Norovirus capsid displays an icosahedral symmetry that is composed of 180 copies of a single major structural protein, the capsid protein (VP1), which organize into 90 dimers. Each VP1 can be divided into two major domains, the N-terminal shell (S) and the C-terminal protruding (P) domains, linked by a short hinge. The P domain is further divided into P1 and P2 subdomains, forming the leg and the head of the protruding P dimer, respectively. Expression of the S domain alone formed smooth, thin-layer S particles without the protruding structures, while production of P domain in vitro resulted in P dimer, P particle, and small P particle. Functional analyses showed that the P dimer and the P particle, but not the S particle, bind to histo-blood group antigens (HBGAs), the host susceptible factors of noroviruses (see below), indicating that the P domain is the HBGA binding domain.

The P domain of VA207 (amino acid 222 to 537) was expressed in E. coli and the HBGA binding profile of the resulting P protein was verified (data not shown) before being used in the crystallography study. The crystal of the native P protein of VA207 belongs to space group of P21212 and contains a homodimer of P protein in an asymmetric unit. Most residues from 226 to 527 could be modeled in the electron density map, while residues 295 to 297 and 392 to 394 could not be modeled due to lack of interpretable electron density map in these loop regions. P2 subdomain, spanning from residue 275 to 415, is an insertion into P1 subdomain, splitting the latter into two fragments (222 to 274 and 416 to 537). While P1 forms the legs, P2 constitutes the head of the P dimer with a β-barrel made of 6 antiparallel β strands folded as a Greek key topology. The P dimer has a dimension of 56 by 66 by 70 Å and contains a large buried surface area of 3, 300 Å2 (for two protomers) formed by both polar and non-polar residues. Both subdomains contributed to the dimer interface: the α helices in the P1 subdomain interacts with each other by hydrogen bonds and hydrophobic interaction, while strands β5 and β9 from the β barrel in P2 subdomain was bound mainly by hydrogen bonds. Similar to the protomers, the general structure of VA207 P dimer is very similar to that of VA387, particularly in the P1 subdomain region. However, significant differences were observed in the four loops on the P2 subdomain connecting β2-β3, β4-β5, β6-β7 and β7-β8, as a result of sequence variations in the four loops between the two strains.

>SKTKAFTIPVLKISEMTNSRFPVPVDQMYTSRSEGIVVQPQNGRATIDGELLGTTLVSPVSVCNFKGNLQAEVPGQHQLYQLQLTNLDGSPIDPTDDTPGPLGCPDFTGLLYGVASQRGPGDATRAHEARIDTGSDTFAPKIGQVRFYSTSSDFETNQPTHFTPIGIYIEGNSSDFNQWQLPRYGGHLANNNHLAPAVSPLFPGEQILFFRSFIPGASGHTNGEMDCLLPQEFVQHFYQEAATARSEVALLRFVNPDTGRALFESKLHKQGFMTIASSGDHPIIMPTNGYFRFEAWVNQFYSLAPVGTGSGRRRIQ[2x]> DWVVAPISVPENGEGPFPQRLNQLKSNKDRDTKIFYSITGPGADSPPEGVF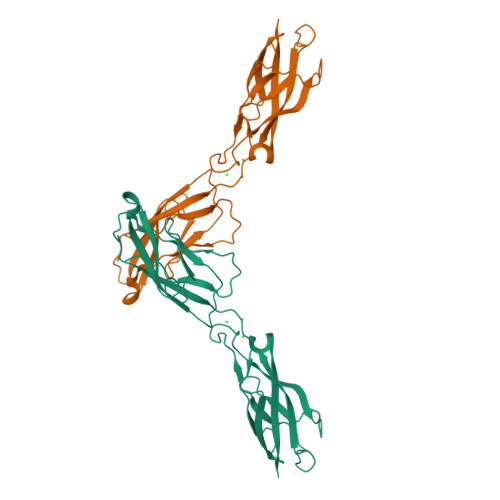AVEKETGWLLLNKPLDREEIAKYELFGHAVSENGASVEDPMNISIIVTDQNDHKPKFTQDTFRGSVLEGVLPGTSVMQVTATDEDDAIYTYNGVVAYSIHSQEPKDPHDLMFTIHRSTGTISVISSGLDREKVPEYTLTIQATDMDGDGSTTTAVAVVEILD>[4x]MTTRLTRWLTALDNFEAKMALLPAVRRYGRLTRATGLVLEATGLQLPLGATCIIERQDGPETKEVESEVVGFNGQRLFLMPLEEVEGILPGARVYARNGHGDGLQSGKQLPLGPALLGRVLDGGGKPLDGLPAPDTLETGALITPPFNPLQRTPIEHVLDTGVRAINALLTVGRGQRMGLFAGSGVGKSVLLGMMARYTRADVIVVGLIGERGREVKDFIENILGPDGRARSVVIAAPADVSPLLRMQGAAYATR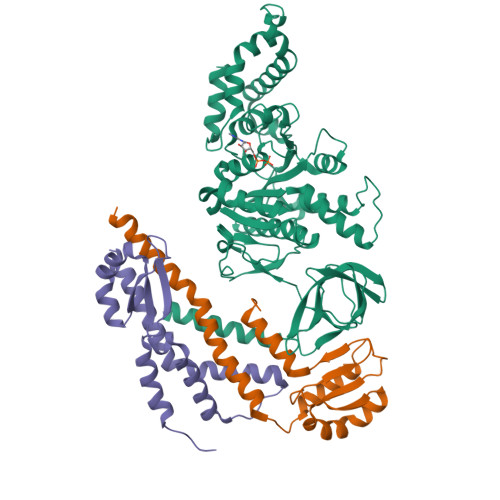IAEDFRDRGQHVLLIMDSLTRYAMAQREIALAIGEPPATKGYPPSVFAKLPALVERAGNGIHGGGSITAFYTVLTEGDDQQDPIADSARAILDGHIVLSRRLAEAGHYPAIDIEASISRAMTALITEQHYARVRLFKQLLSSFQRNRDLVSVGAYAKGSDPMLDKAITLWPQLEAFLQQGIFERADWEDSLQALDLIFPTV;>GSHAPIHARMQQLVSEFQNTLDALDSVIASRLMQMALEAARQVIGQTPAVDNSALIKQIQQLLQQEPLFSGKPQLRVHPDDLQRVEEMLGATLSLHGWRLRGDPTLHHGGCKVSADEGDLDASVATRWQELCRLAAPGVL[8x]>[2x]MYQAGGTIRSLLDKVAEQEYLLPAIQREFVWRPEQICRLFDSLLQGYPFGTFLFWKIKPENRDSYQFYQFMQHYHERDNYHCENVTQLPEREFIAVLDGQQRITALNIGLRGSFAWKLTGKWWSNDDAFPVRRLHLNLLSKPDLETGSMYDFEFLTDDKASLDASEQYWFRVGRIMEEEEDALIDEVADDARLSSEQRKEARSTLRHLYRTIHDKDKISFYEESDQSLERVLNIFIRMNSGGTTLSYSDLLLSIAVAQWSSLDAREEIHALVDEMNRVGDGFNVSKDLVLKAGLMLSDIGSVGFKVENFNKENMAILEKNWTPIRDALLLSMQLLASFGFNAQNLRATSAILPLAYYLHHRKLTASYLSRVEYA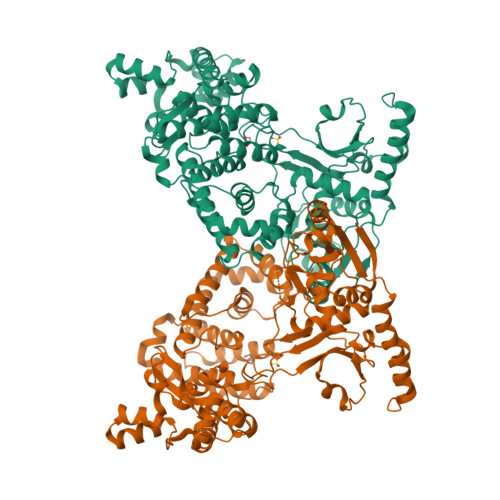VDRECIRNWLIRSLLKASGIWGSGLDTLLTMLRSDIKQSGDTGFPLAKIEATMQQRGKSLRFDPEEISELAQLDYGNPRTFALLTLLFPGFDFSRHFHVDHIYPKGLFTRNKLAKVGVPAEQLDELIEASNKLPNLQLLEGTINNQKRQKMPHEWYAQQWPDVNARQAHLQSQAITSLPEQLNQFMDFYRERQETLLARIRTALQPASSVETE> GPKYTMFHYLRAQEFEHGKSRIALTNSVNEALLNPSRVYTFFSSDYVKKVNKATEAAMFLGWVEQLVYDFTDETSEVSTTDKIADITIIIPYIGPALNIGNMLYKDDFVGALIESGAVILLEFIPEIAIPVLGTF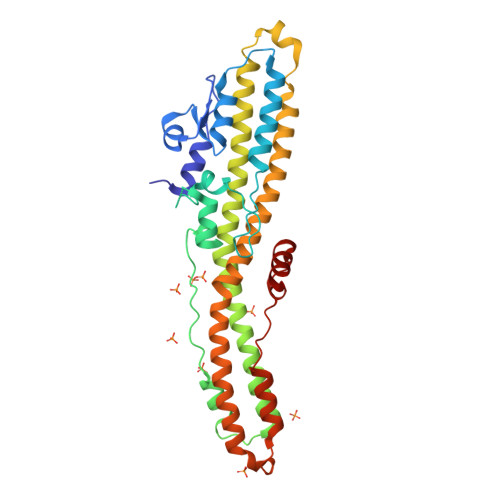ALVSYIANKVLTVQTIDNALSKRNEKWDEVYKYIVTNWLAKVNTQIDLIRKKMKEALENQAEATKAIINYQYNQYTEEEKNNINFNIDDLSSKLNESINKAMININKFLNQCSVSYLMNSMIPYGVKRLEDFDASLKDALLKYIYDNRGTLIGQVDRLKDKVNNTLSTDIPFQLSKYVDNQRLLSTFTEYIK>[2x]GPLGSMAAAPPLRDRLSFLHRLPILLKGTSDDDVPCPGYLFEEIAKISHESPGSSQCLLEYLLSRLHSSSGHGKLKVLKILLYL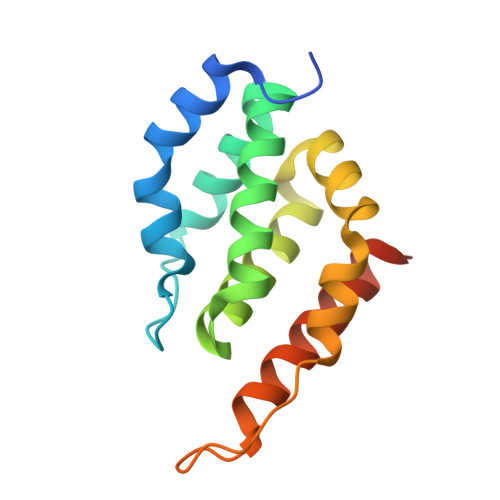CSHGSSFFLLILKRNSAFIQEAAAFAGPPDPLHGNSLYQKVRAAAQDLGSTLFSDTVLPLA>MELQEVLRMNGGEGDTSYAKNSAYNQLVLAKVKPVLEQCVRELLRANLPNINKCIKVADLGCASGPNTLLTVR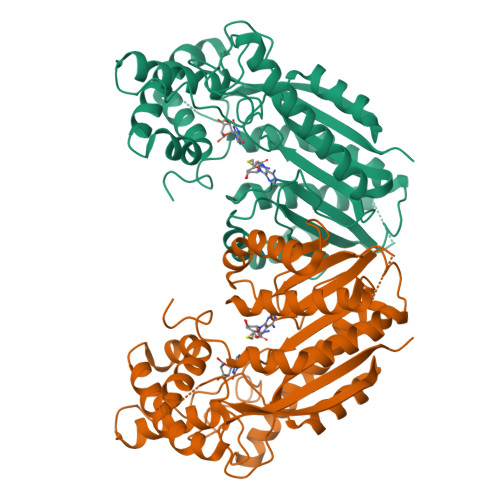DIVQSIDKVGQEKKNELERPTIQIFLNDLFPNDFNSVFKLLPSFYRKLEKENGRKIGSCLIGAMPGSFYSRLFPEESMHFLHSCYCLQWLSQVPSGLVTELGIGTNKGSIYSSKASRLPVQKAYLDQFTKDFTTFLRIHSEELFSHGRMLLTCICKGVELDARNAIDLLEMAINDLVVEGHLEEEKLDSFNLPVYIPSAEEVKCIVEEEGSFEILYLETFKVLYDAGFSIDDEHIKAEYVASSVRAVYEPILASHFGEAIIPDIFHRFAKHAAKVLPLGKGFYNNLIISLAKKPEKSDM[4x]>MEVEKTACPSGKKAREIDESLIFYKKWELEACVDAALLATQMDRVNAIPFTYEQLDVLKHKLDELYPQGYPESVIQHLGYLFLKMSPEDIRKWNVTSLETLKALLEVNKGHEMSPQVATLIDRFVKGRGQLDKDTLDTLTAFYPGYLCSLSPEELSSVPPSSIWAVRPQDLDTCDPRQLDVLYPKARLAFQNMNGS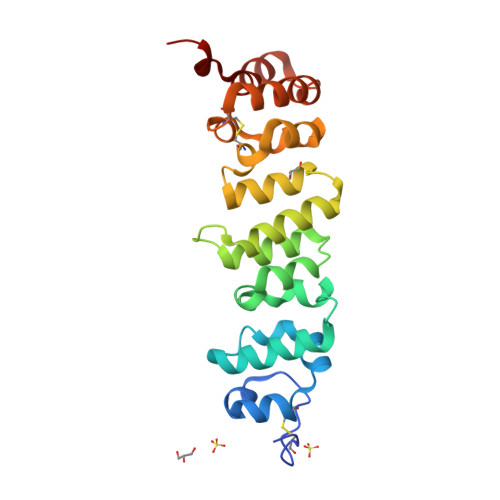EYFVKIQSFLGHHHHHH[2x]LORACABEF (Open form) | C16 H18 Cl N3 O4 | 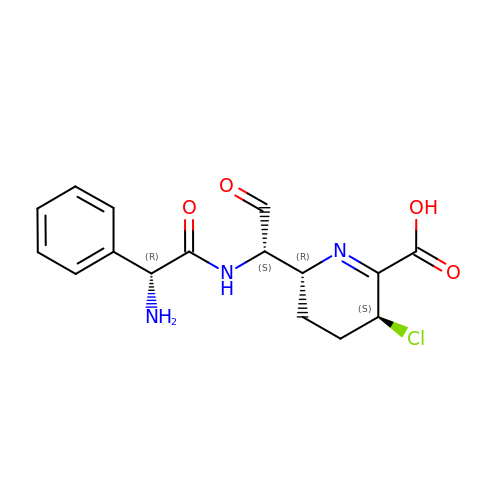DRTWKGBDHBOYMS-UMSGYPCISA-N> GPLGSMENSCNFNNSIKNVIVFYINEKALIEEKKMLSCYENKLLNLIKEDCENIMLKYKPNLSYICSLLKVDDTSEENIKHIKDQIIESLENDNRPSVKLAIISLISMIVEM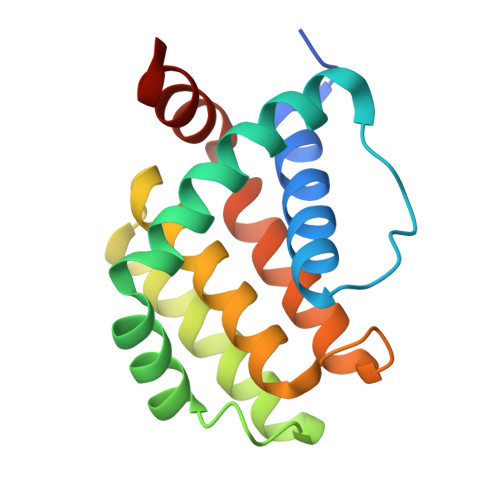NGYKGKNIPMSFLIEDIALKISENSEDLINFINIKNKQKS> ANIVGGIEYSI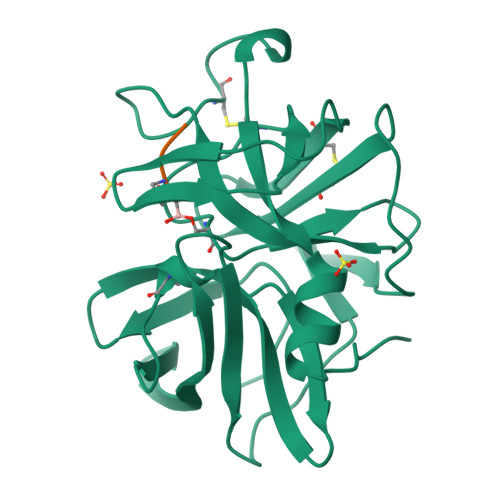NNASLCSVGFSVTRGATKGFVTAGHCGTVNATARIGGAVVGTFAARVFPGNDRAWVSLTSAQTLLPRVANGSSFVTVRGSTEAAVGAAVCRSGRTTGYQCGTITAKNVTANYAEGAVRGLTQGNACAGRGDSGGSWITSAGQAQGVMSGANVQSNGNNCGIPASQRSSLFERLQPILSQYGLSLVTG;> XAAPA>[4x]MNVVVIGGGAAGLKAASRIRRKDGDASITVVEAGKYVSLGRCGLPYYVGGLVHEVDNLRETTYGAVRDEAYFKKLKNIDVLTETVATEIDRSRKTVKIVRNGSEDELNYDYLVIATGARPAKPPIEGIEAEGVVTLTSAEEAEKIIEMWEEGAEKAVVIGAGFIGLESAEALKNLDMEVTVIEMMDRVAPAMLDREMAVLVENHLREKGVNVVTSTRVEKIVSQDDKVRAVIANGKEYPADVVVVATGIKPNSELAEKAGLKIGETGAIWVDEYMRTSDESIYAGGDCVETTCLVTGKKIIAPFGDVANKQGRVIGENITGGRAVFPGVIRTAIFKVFDFTAASAGVNEQMAKEAGLDYFTVIAPSPDRAHYYPQANYIRLKLIVEKGSWRVIGAQGVGMGEVAKRIDVLSTAIQAGMTIDQLANLDLAYAPPYSPALDPVITIANVAMNKRDGLFEGINVFELKEKLEKEDIVILDVRSEEEFKTRRIESEKVIHIPILELRERLDEIPRDKEIVVVCAIGLRSFEASRILKHAGFEKVKILEGGMAFWF

NADH-dependent persulfide reductase (Npsr) has been proposed to facilitate dissimilatory sulfur respiration by reducing persulfide or sulfane sulfur-containing substrates to H2S. Pyridine nucleotide disulfide oxidoreductases (PNDORs) are a large class of homodimeric NADH- and FAD-dependent enzymes that generally function to reduce small molecule substrates at a catalytic cysteine positioned at the si face of the isoalloxazine ring. The major structural difference between CoADR and Npsr is the addition of a ~100-amino acid rhodanese-like domain to the C-terminus of the Npsr. A surface-accessible cysteine in this domain serves as the initial sulfur-accepting site before a molecule of CoA bound to the FAD-containing domain chaperones the sulfur to the active site cysteine adjacent to FAD.

The 3.1 Å X-ray structure of AfNpsr reveals access to the tightly bound catalytic CoA, and the active site Cys 42 is restricted by a flexible loop (residues 60-66) that is not seen in the bacterial homologs from Shewanella loihica PV-4 and Bacillus anthracis. As expected, the enzyme is a dimer, with the N-terminal FAD-binding domain (residues 1-448) having nearly identical topology to related Npsr and CoADR proteins. Residues 449 through 550 make up the C-terminal rhodanese domain, which is linked to the FAD domain by a single amino acid chain. On all four AfNpsr subunits found in the asymmetric unit, two loops on the rhodanese domain comprising residues 465-472 and 483-488 were missing due to disorder. In AfNpsr, CoA is deeply buried, and in this configuration of the protein, CoA has little access to the solvent except for a small opening above the pantothenic acid arm. In AfNpsr, the seemingly low accessibility of CoA from the surface of the protein results from a larger loop consisting of residues 60-66 (TTYGAVR) that closes over the CoA binding pocket. It should be noted that for the dimer with the ordered loop, the average B-factor for the loop is 67 Å2 compared to 47 Å2 for the rest of the FAD-binding domain, suggesting there is some flexibility for the opening and closing of the loop over the enzyme-bound CoA. For NADP+, the phosphorylated 2′ hydroxyl group of ribose introduces steric clashes with E183, M184, and M185 as well as strong electrostatic repulsions with E183. A metal ion binding site is located 5.2 Å from FAD. Given that AfNpsr has all of the same catalytic components as the other Npsr and CoADR homologs and that none of these have any demonstrated metal dependence, it is likely that the bound metal ion in AfNpsr plays a structural role.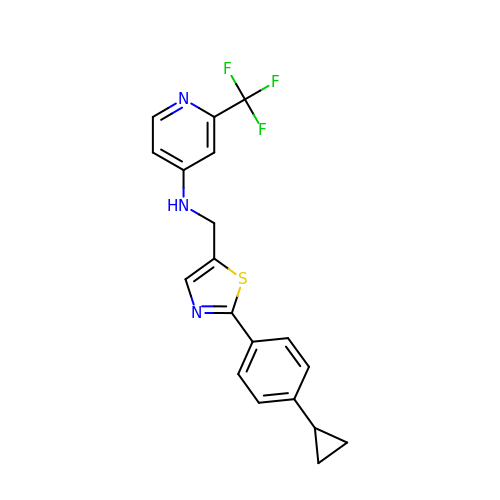~{N}-[[2-(4-cyclopropylphenyl)-1,3-thiazol-5-yl]methyl]-2-(trifluoromethyl)pyridin-4-amine | C19 H16 F3 N3 S | MNFFCZFIFAZOEV-UHFFFAOYSA-N> QTEMDKVNVDLAAAGV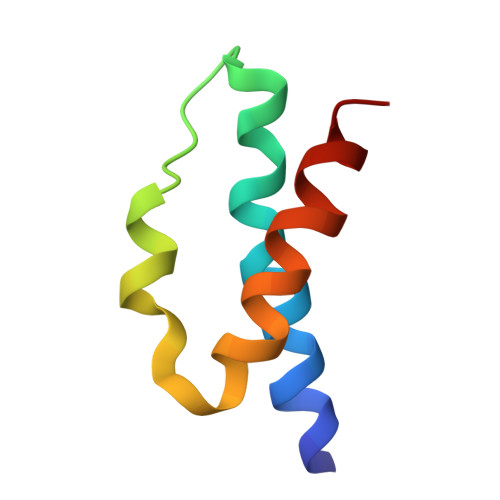AFKERYNMPVIAEAVEREQPEHLRSWFRERLIAHRLASVN>MNVVIVRYGEIGTKSRQTRSWFEKILMNNIREALVTEEVPYKEIFSRHGRIIVKTNSPKEAANVLVRVFGIVSISPAMEVEASLEKINRTALLMFRKKAKEVGKERPKFRVTARRITKEFPLDSLEIQAKVGEYILNNENCEVDLKNYDIEIGI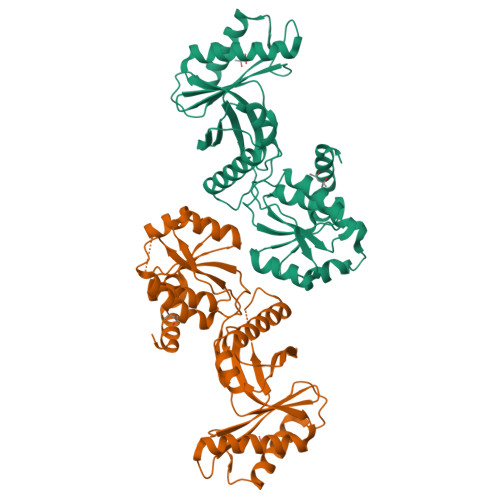EIMQGKAYIYTEKIKGWGGLPIGTEGRMIGILHDELSALAIFLMMKRGVEVIPVYIGKDDKNLEKVRSLWNLLKRYSYGSKGFLVVAESFDRVLKLIRDFGVKGVIKGLRPNDLNSEVSEITEDFKMFPVPVYYPLIALPEEYIKSVKERLGL[2x]> MNQEEAIFRSADMTYVQLYIPLEVIREVTFLLGKMSVFMVMDLNKDLTAFQRGYVNQLRRFDEVERMVGFLNEVVEKHAAETWKYILHIDDEGNDIAQPDMADLINTMEPLSLENVNDMVKEITDCESRARQLDESLDSLRSKLNDLLEQRQVIFECSKFIEVNPGIAGRATNPEIEQEERDVDEFRMTPDDISETLSDAFSFDDETPQDRGALGNDLTRNQSVEDLSFLEQGYQHRYMITGSIRRTKVDILNRILWRLLRGNLIFQNFPIEEPLLEGKEKVEKDCFIIFTHGETLLKKVKRVIDSLNGKIVSLNTRSSELVDTLNRQIDDLQRILDTTEQTLHTELLVIHDQLPVWSAMTKREKYVYTTLNKFQQESQGLIAEGWVPSTELIHLQDSLKDYIETLGSEY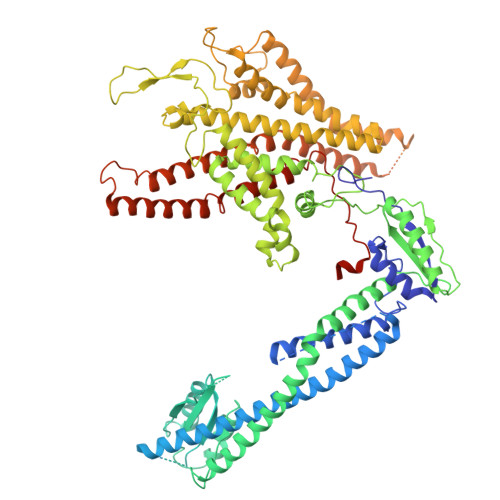STVFNVILTNKLPPTYHRTNKFTQAFQSIVDAYGIATYKEINAGLATVVTFPFMFAIMFGDMGHGFILFLMALFLVLNERKFGAMHRDEIFDMAFTGRYVLLLMGAFSVYTGLLYNDIFSKSMTIFKSGWQWPSTFRKGESIEAKKTGVYPFGLDFAWHGTDNGLLFSNSYKMKLSILMGYAHMTYSFMFSYINYRAKNSKVDIIGNFIPGLVFMQSIFGYLSWAIVYKWSKDWIKDDKPAPGLLNMLINMFLAPGTIDDQLYSGQAKLQVVLLLAALVCVPWLLLYKPLTLRRLNKNGGGGRPHGYQSVGNIEHEEQIAQQRHSAEGFQGMIISDVASVADSINESVGGGEQGPFNFGDVMIHQVIHTIEFCLNCISHTASYLRLWALSLAHAQLSSVLWDMTISNAFSSKNSGSPLAVMKVVFLFAMWFVLTVCILVFMEGTSAMLHALRLHWVEAMSKFFEGEGYAYEPFSFRAIIEDYKDHDGDYKDHDIDYKDDDDK> MNPVTKQFQFGQSTVTLETGRIARQATGAVLVTMDDVSVLVTVVGAKSPAEGRDFFPLSVHYQEKTYAAGRIPGGFFKREGRPSEKETLTSRLIDRPIRPLFPEGFMNEVQVVCTVVSTNKKSDPDIAAMIGTSAALAISGIPFAGPIGAARVGFHPEIGYI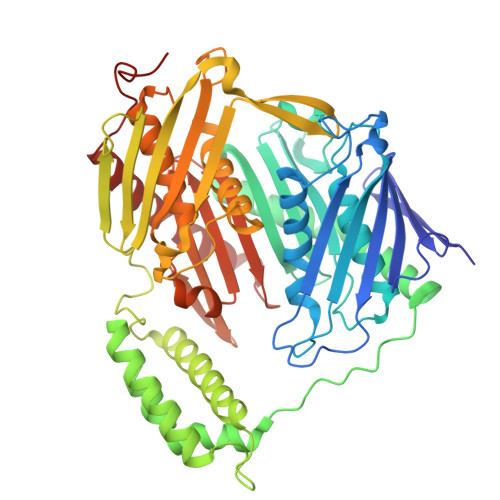LNPTYEQLQSSSLDMVVAGTEDAVLMVESEADELTEDQMLGAVLFAHDEFQAVIRAVKELAAEAGKPAWDWKAPAENTVLVNAIKAELGEAISQAYTITIKQDRYNRLGELRDQAVALFAGEEEGKFPASEVKDVFGLLEYRTVRENIVNGKPRIDGRDTRTVRPLRIEVGVLGKTHGSALFTRGETQALVVATLGTARDAQLLDTLEGERKDAFMLHYNFPPFSVGECGRMGSPGRREIGHGRLARRGVAAMLPTQDEFPYTIRVVSEITESNGSSSMASVCGASLALMDAGVPVKAPVAGIAMGLVKEGEKFAVLTDILGDEDHLGDMDFKVAGTDKGVTALQMDIKINGITEEIMEIALGQALEARLNILGQMNQVIAKPRAELSENAP[(2R,3S,4R,5R)-5-(2-amino-6-oxo-1,6-dihydro-9H-purin-9-yl)-3,4-dihydroxytetrahydrofuran-2-yl]methyl (2R,3S,4R,5S,6R)-3,4,5-trihydroxy-6-(trifluoromethyl)tetrahydro-2H-pyran-2-yl dihydrogen diphosphate (non-preferred name) | C16 H22 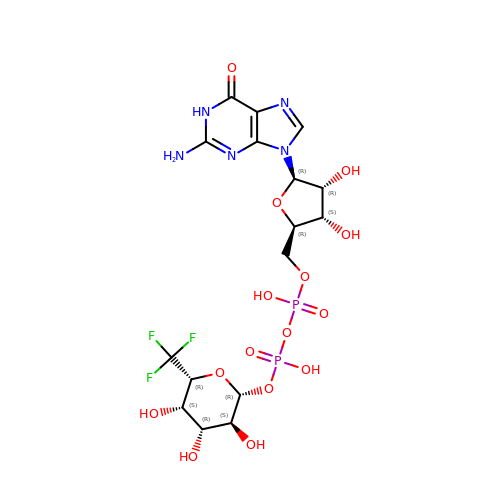F3 N5 O15 P2 | CBLFMUIUVZLPER-KLZHJQHWSA-N> GHMKQEELKRLYKAQAIQRQLEEVEERQRASEIQGVRLEKALRGEADSGTQDEAQLLQEWFKLVLEKNKLMRYESELLIMAQELELEDHQSRLEQKLREKMLKEESQKDEKDLNEEQEVFTEL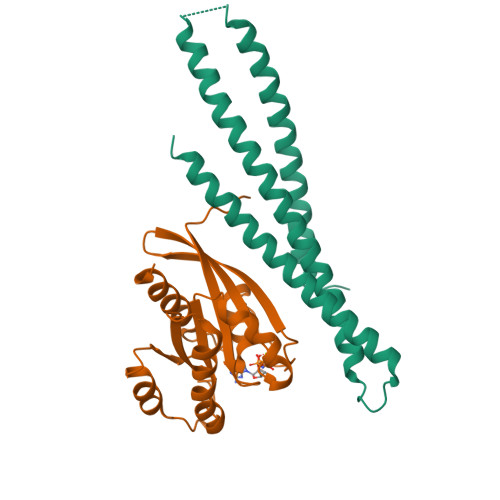MQVIEQRDKLVDSLEEQRIREKAEDQHFES;> GHMAKTYDYLFKLLLIGDSGVGKSCLLLRFADDTYTESYISTIGVDFKIRTIELDGKTIKLQIWDTAGQERFRTITSSYYRGAHGIIVVYDVTDQESYANVKQWLQEIDRYASENVNKLLVGNKSDLTTKKVVDNTTAKEFADSLGIPFLETSAKNATNVEQAFMTMAAEIKKRMGPGAASGGERPNLKIDSTPVKPAGGGCC>[2x]MAGKKVLIVYAHQEPKSFNGSLK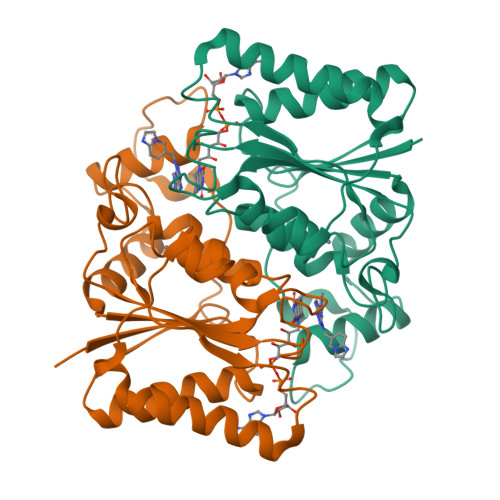NVAVDELSRQGCTVTVSDLYAMNLEPRATDKDITGTLSNPEVFNYGVETHEAYKQRSLASDITDEQKKVREADLVIFQFPLYWFSVPAILKGWMDRVLCQGFAFDIPGFYDSGLLQGKLALLSVTTGGTAEMYTKTGVNGDSRYFLWPLQHGTLHFCGFKVLAPQISFAPEIASEEERKGMVAAWSQRLQTIWKEEPIPCTAHWHFGQHHHHHH> GSVSKWSTDEVSEFIQSLPGCEEHGKVFKDEQIDGEA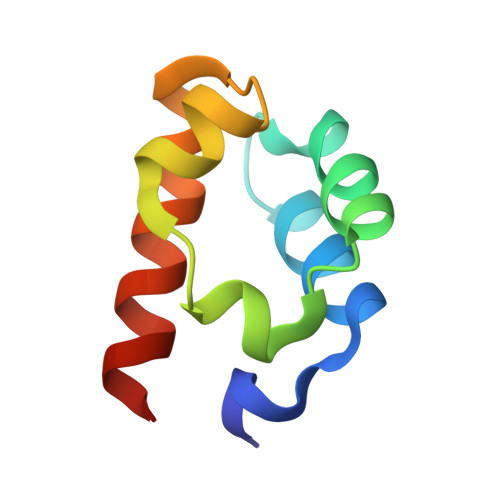FLLMTQTDIVKIMSIKEGPAEKIFNSILMFKAAEKN>[60x]GSGVGISTGGWVGGSHFADKYVITKNTRQFITSIQNGHLYKTEIINPSNGNGKSQRCVTTPWTYFNFNQYSCHFSPQDWQRLTNEYKRFRPKAMLVKIYNLQIKQILSNGADTTYNNDLTAGVHIFCDGEHAYPNASHPWDEDVMPDLPYKTWKLFQYGYIPILNELADLDGTTAGGTATEKAILYQMPFFMLENSDHEVLRTGESSEFTFNFDCEWVNNERAYIPPGLMFNPKVPTRRVQYIRQNGQTTASTSRIEPYSKPTSWMTGPGFLGGQRVGPATSDTAPYMVCTKPDGVYINTGAAGYGSGFDPPSGSLAPTDLEYKLQWYQTPEDTGNNGNIIANPSLSMLRDQLLYRGNQTTYNLNADVWMFPNQIWDRYPITREHPIWCKKPRADKNTIIDPFDGSIAMDHPPGTIFIKMAKIPVPSSTNADSYLNIYCTGQVSCEIVWEVERYVTKNWRPERRHTALGMSIGGTENVSPTYHVDSAGTYIQPTTFDQCMPVKTNINKVL

Gorilla bocavirus 1 (GBoV1) is a member of the genus Bocaparvovirus in the Parvoviridae that contain single-stranded DNA (ssDNA) packaging viruses. The structural proteins that form the viral capsid, VP1, VP2 and VP3, are encoded by the cap gene. Sixty copies of VP1, VP2 and VP3 assemble one T = 1 icosahedral capsid in an approximate 1:1:10 ratio in 2-, 3-, 5-related symmetries. GBoV1 is an alternative to HBoV1, as it is capable of also infecting the apical side of pHAE efficiently, package 5.5 kb and less susceptible to neutralization by pooled intravenous immunoglobulin (IVIgs).

3D image reconstruction of 168,565 GBoV1 WT and 218,746 GBoV1 VP3-only capsids resulted in structures with an estimated resolution of 2.76 Å for both types of capsids based on an FSC threshold of 0.143. The GBoV1 capsid structures were identical, despite being assembled from different VP compositions. They share the conserved features of the Parvoviridae subfamily, with a channel at the 5-fold symmetry axis, protrusions around the 3-fold axis, the 2/5-fold wall, located between the depressions at the 2- and 5-fold axes and depressions at the 2-fold as well as around the 5-fold axis. The basket-like structure beneath the 5-fold channel previously reported within the capsids of HBoV1-HBoV4 and BPV, was less pronounced in GBoV1 suggesting less order at the N-terminus of the VP. In both the GBoV1 structures, excluding residues 1–32, residue 33 to the last C-terminal residue, aa542 (VP3 numbering), were structurally ordered and models could be built into the cryo-reconstructed density maps. The GBoV1 VP3 structure conserved the parvovirus features, including the eight-stranded β-barrel motif, α-helix A and β-strand A. The structure also featured α-helix B, a region unique to the bocaparvoviruses and the ten defined VRs, VR-I to VRVIIIB and VR-IX. In addition to the high-resolution WT structure, the structures of two capsid-antibody complex structures are reported, highlighting antigenic epitopes on the GBoV1 capsid surface. Both, GBoV1 and HBoV1 share a high sequence and structural identity, with major structural differences localized to VR-I, VR-III and VR-V. VR-I and VR-III are both part of the 2/5-fold wall of the capsid and VR-V is located on the protrusions around the icosahedral 3-fold. The 15C6 epitope lines the 5-fold channel, encompassing the residues that form VR-II (residues 142-GAD-144) and VR-VIIIB (residues 460-STNA-463), which are the DE and HI loops, respectively. The 12C1 epitope sits on the protrusions around the 3-fold axis and contains contact residues from VR-I (80-SNGN-83), VR-IV (276-IRQNGQTTA-284) and VR-VIII (390-NQTT-393).1,3-BIS-([3-(4-{3-[3-NITRO-5-(GALACTOPYRANOSYLOXY)-BENZOYLAMINO]-PROPYL}-PIPERAZIN-1-YL)-PROPYL-AMINO]-CARBONYLOXY)-2-AMINO-PROPANE 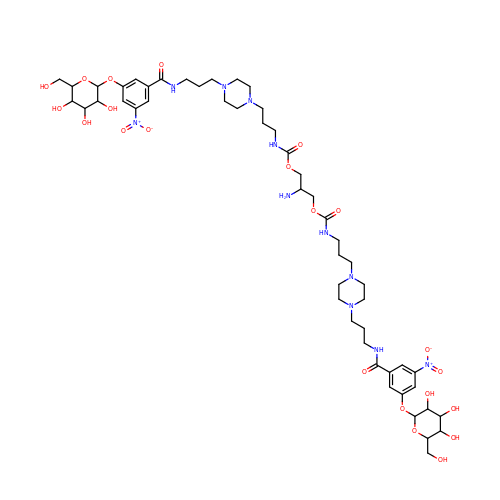| C51 H79 N11 O22 | RJLCAAJYVGPDFG-LNGNCPBTSA-N>MRLCIPQVLLALFLSMLTAPGEGSRRRATQARDTTQPALLRLSDHLLANYKKGVRPVRDWRKPTTVSIDVIMYAILNVDEKNQVLTTYIWYRQYWTDEFLQWTPEDFDNVTKLSIPTDSIWVPDILINEFVDVGKSPNIPYVYVHHRGEVQNYKPLQLVTACSLDIYNFPFDVQNCSLTFTSWLHTIQDINITLWRSPEEVRSDKSIFINQGEWELLEVFPQFKEFSIDISNSYAEMKFYVIIRRRPLFYAVSLLLPSIFLMVVDIVGFCLPPDSGERVSFKITLLLGYSVFLIIVSDTLPATAIGTPLIGVYFVVCMALLVISLAETIFIVRLVHKQDLQRPVPDWLRHLVLDRIAWILCLGEQPMAHRPPATFQANKTDDCSGSDLLPAMGNHCSHVGGPQDLEKTPRGRGSPLPPPREASLAVRGLLQELSSIRHFLEKRDEMREVARDWLRVGYVLDRLLFRIYLLAVLAYSITLVTLWSIWHYS[5x]

5-HT3Rs are expressed either as a homopentamer consisting of subunit A or as heteropentamers of subunit A in combination with other subunits (B, C, D, or E). 5-HT3Rs are widely expressed in both the central and peripheral nervous system, and form a part of the brain–gut circuitry that directly control peristalsis, emetic reflex, and visceral pain perception. The 5-HT3R antagonists, referred to as “setrons,” are the standard first line of therapy for the prevention of chemotherapy-induced emesis. Granisetron is a competitive antagonist that inhibits serotonin-activated currents at nanomolar concentrations.

In the present study, we have solved the structure of the full-length 5-HT3AR bound to granisetron at 2.92 Å resolution. According to this 5-HT3AR-granisetron structure, residues from loops A, B, and C on the principal (+) subunit and loops D, E, and F from the complementary (−) subunit form an enclosure around granisetron. The cationic center of granisetron is a tertiary ammonium in the bicyclic ring (pKa 9.6) and is positioned at the deep end of the pocket nestled by Trp156 (loop B), Tyr207 (loop C), Trp63 (loop D), and Tyr126 (loop E). However, in comparison to serotonin, granisetron is larger in size and extends further outward into the subunit interface such that the aromatic indazole ring is oriented parallel to the membrane and makes a cation–pi interaction with the positively charged nitrogen in the guanidinium group of Arg65. Granisetron’s position also requires Arg65 (loop D) and Trp168 (loop F) side chains to reorient. Instead, an alignment of 5-HT3AR-granisetron with the 5-HT3AR-apo structure shows a counter-clockwise twist of β- strands in the ECD, leading to a small inward movement of loop C closing in on granisetron. The loop C conformation in 5-HT3AR-granisetron, although open, is distinct from other antagonist loop C conformations because it lies between the open position of loop C in the 5-HT3AR-apo structure and the closed position in the 5-HT3AR-serotonin structure. The TMD of 5-HT3AR-granisetron is rotated clockwise compared to 5-HT3AR-apo, once again in a position between the apo and serotonin-bound structures. Although granisetron induces a rotational movement in the TMD, the pore radius is comparable to 5-HT3AR-apo and the permeation pathway presents barriers in all the three domains. Thus, the 5-HT3AR-granisetron structure represents a non-conducting conformation.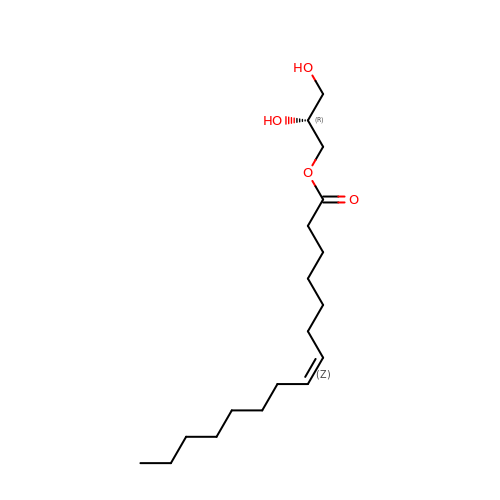(2R)-2,3-DIHYDROXYPROPYL(7Z)-PENTADEC-7-ENOATE | C18 H34 O4 | BJMLBVHMHXYQFS-XZVRFQMRSA-N> ADTVTLPFANGERPLVMYPGKRPLIGLTARPPQLETPFSVFDEGLITP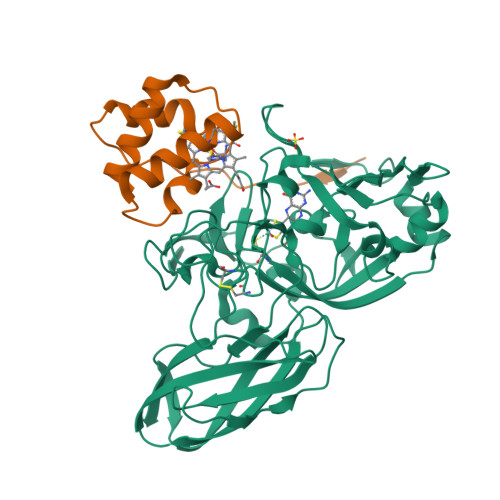NDAFFVRYHLAGIPLEIDPDAFRLEIKGKVGTPLSLSLQDLKNDFPASEVVAVNQCSGNSRGFVEPRVGGGQLANGAMGNARWRGVPLKAVLEKAGVQAGAKQVTFGGLDGPVIPETPDFVKALSIDHATDGEVMLAYSMNGADLPWLNGYPLRLVVPGYYGTYWVKHLNEITVIDKEFDGFWMKTAYRIPDNACACTEPGKAPTATIPINRFDVRSFITNVENGASVKAGEVPLRGIAFDGGYGITQVSVSADAGKSWTNATLDPGLGKYSFRGWKAVLPLTKGDHVLMCRATNARGETQPMQATWNPAGYMRNVVEATRVIAA;> APLTYELPDETAQLKPAPQPGFEAAQNNCAACHSVDYINTQPPGKGQAFWDAEVQKMIKVYHAPVDEADAKAIADYLAKTY> GSMADEATRRVVSEIPVLKTNAGPRDRELWVQRLKEEYQSLIRYVENNKNADNDWFRLESNKEGTRWFGKCWYIHDLLKYEFDIEFDIPITYPTTAPEIAVPELDGKTAKMYRGGKIELTDHFKPLWARNVPKFGLAHLMALGLGP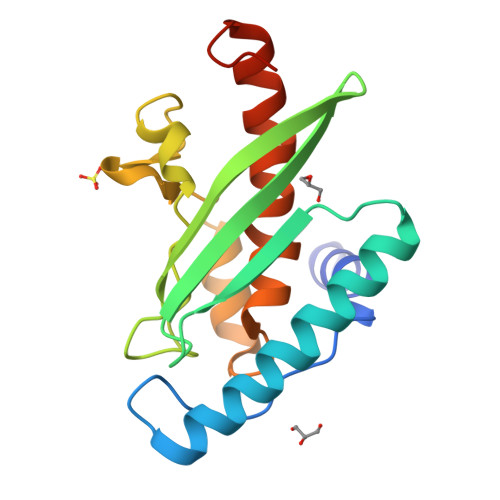WLAVEIPDLIQKGVIHHKEKCNQ>MAYTTAQLVTAYTNANLGKAPDAATTLTLDAYATQTQTGGLSDAAALTNTLKLVNSTTAVAIQTYQFFTGVAPSAAGLDFLVDSTTNTNDLNDAYYSKFAQENRFINFSINLATGAGAGATAFAAAYTGVSYAQTVATAYDKIIGNAVATAAGVDVAAAVAFLSRQANIDYLTAFVRANTPFTAAADIDLAVKAALIGTILNAATVSGIGGYATATAAMINDLSDGALSTDNAAGVNLFTAYPSSGVSGSTLSLTTGTDTLTGTANNDTFVAGEVAGAATLTVGDTLSGGAGTDVLNWVQAAAVTALPTGVTISGIETMNVTSGAAITLNTSSGVTGLTALNTNTSGAAQTVTAGAGQNLTATTAAQAANNVAVDGGANVTVASTGVTSGTTTVGANSAASGTVSVSVANSSTTTTGAIAVTGGTAVTVAQTAGNAVNTTLTQADVTVTGNSSTTAVTVTQTAAATAGATVAGRVNGAVTITDSAAASATTAGKIATVTLGSFGAATIDSSALTTVNLSGTGTSLGIGRGALTATPTANTLTLNVNGLTTTGAITDSEAAADDGFTTINIAGSTASSTIASLVAADATTLNISGDARVTITSHTAAALTGITVTNSVGATLGAELATGLVFTGGAGADSILLGATTKAIVMGAGDDTVTVSSATLGAGGSVNGGDGTDVLVANVNGSSFSADPAFGGFETLRVAGAAAQGSHNANGFTALQLGATAGATTFTNVAVNVGLTVLAAPTGTTTVTLANATGTSDVFNLTLSSSAALAAGTVALAGVETVNIAATDTNTTAHVDTLTLQATSAKSIVVTGNAGLNLTNTGNTAVTSFDASAVTGTGSAVTFVSANTTVGEVVTIRGGAGADSLTGSATA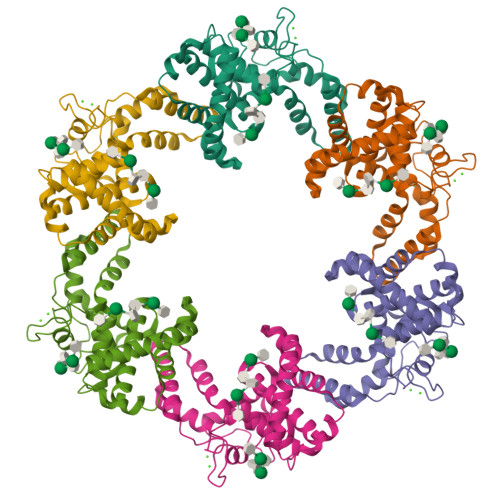NDTIIGGAGADTLVYTGGTDTFTGGTGADIFDINAIGTSTAFVTITDAAVGDKLDLVGISTNGAIADGAFGAAVTLGAAATLAQYLDAAAAGDGSGTSVAKWFQFGGDTYVVVDSSAGATFVSGADAVIKLTGLVTLTTSAFATEVLTLA[6x]>[7x]MIPVTEFRQFSEQQPAFRVLKPWWDVFTDYLSVAMLMIGVFGCTLQVMQDKIICLPKRVQPAQNHSSLSNVSQAVASTTPLPPPKPSPANPITVEMKGLKTDLDLQQYSFINQMCYERALHWYAKYFPYLVLIHTLVFMLCSNFWFKFPGSSSKIEHFISILGKCFDSPWTTRALSEVSGEDSDPKPAFSKMNGSMDKKSSTVSEDVEGSLVNSQSLKSIPEKFVVDKSTAGALDKKEGEQAKALFEKVKKFRLHVEEGDILYAMYVRQTVLKVIKFLIIIAYNSALVSKVQFTVDCNVD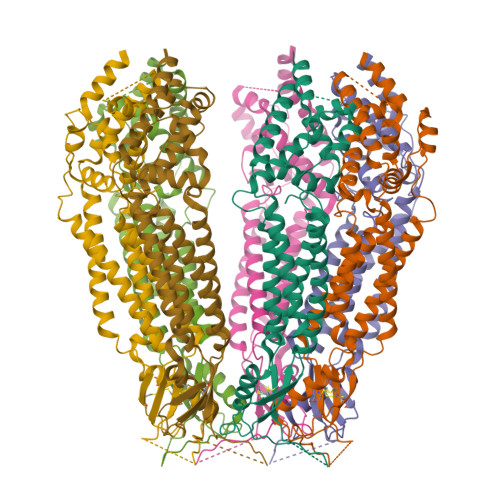IQDMTGYKNFSCNHTMAHLFSKLSFCYLCFVSIYGLTCLYTLYWLFYRSLREYSFEYVRQETGIDDIPDVKNDFAFMLHMIDQYDPLYSKRFAVFLSEVSENKLKQLNLNNEWTPDKLRQKLQTNAHNRLELPLIMLSGLPDTVFEITELQSLKLEIIKNVMIPATIAQLDNLQELSLHQCSVKIHSAALSFLKENLKVLSVKFDDMRELPPWMYGLRNLEELYLVGSLSHDISRNVTLESLRDLKSLKILSIKSNVSKIPQAVVDVSSHLQKMCIHNDGTKLVMLNNLKKMTNLTELELVHCDLERIPHAVFSLLSLQELDLKENNLKSIEEIVSFQHLRKLTVLKLWHNSITYIPEHIKKLTSLERLSFSHNKIEVLPSHLFLCNKIRYLDLSYNDIRFIPPEIGVLQSLQYFSITCNVESLPDELYFCKKLKTLKIGKNSLSVLSPKIGNLLFLSYLDVKGNHFEILPPELGDCRALKRAGLVVEDALFETLPSDVREQMKTEENLYFQGAAAGDYKDDDDK> MDPQGDAAQKTDT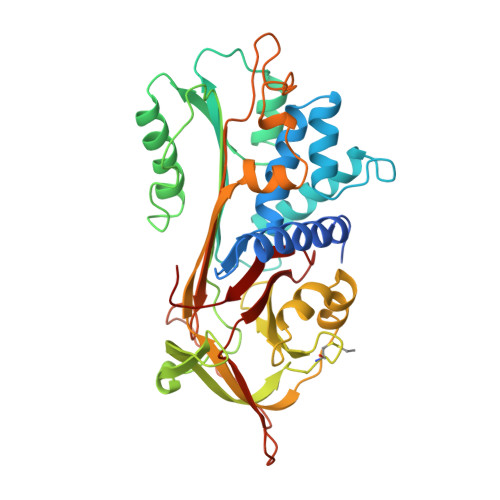SHHDQDHPTFNKITPNLAEFAFSLYRQLAHQSNSTNILFSPVSIATAFAMLSLGTKADTHDEILEGLNFNLTEIPEAQIHEGFQELLRTLNQPDSQLQLTTGNGLFLSEGLKLVDKFLEDVKKLYHSEAFTVNFGDTEEAKKQINDYVEKGTQGKIVDLVKELDRDTVFALVNYIFFKGKWERPFEVKDTEEEDFHVDQVTTVKVPMMKRLGMFNIQHCKKLSSWVLLMKYLGNATAIFFLPDEGKLQHLENELTHDIITKFLENEDRRSASLHLPKLSITGTYDLKSVLGQLGITKVFSNGADLSGVTEEAPLKLSKAVHKAVLTIDEKGTEAAGAMFLEAIPMSIPPEVKFNKPFVFLMIEQNTKSPLFMGKVVNPTQK>SMPDLLTNVAENYVNQDLFAGIEWRIDQDGKPIFQGCAGVKDIETRTFIPKNAIYRIYSMTKPIVSFLAMMLIERGVFRLSSPIQNFDPRFKSMKVIDQHAHIEPATALITIEHLLTHQAGFSYDFSLGCPISAHYRDAQLIEDGGRDLTDMMGVLAELPLVFHPGTQWKYSISTDVLAHIIECATGERVDDLLQRLIFDPLDMQDTGFSLPLDGASRLMEVYGMRSLHGLPALKPAPHVLVPADLGSSHPTDDPDFRRGGHGLYSTLDDYMAFANMLLSGQTPEGETLLSPAVLKLALAPRVHFGARGMRINDEPFAGYSWNLLGRVMTD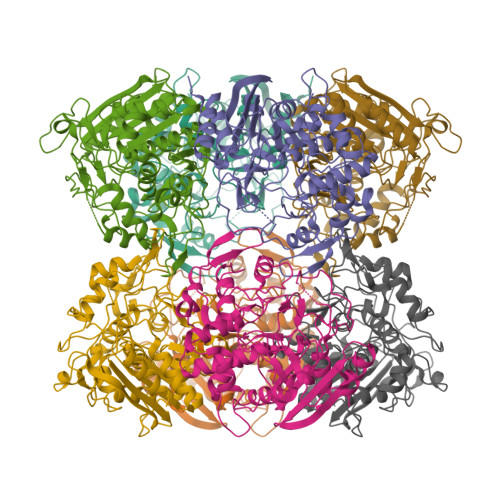VGAAAYATHLGEFGWSGAAATYFWVDPTKNMTGCVMTQFLGSQHPIGSDMQAAAMSMLG[2x]(2Z)-3-(3-chlorobenzyl)-2-imino-5,5-dimethylimidazolidin-4-one 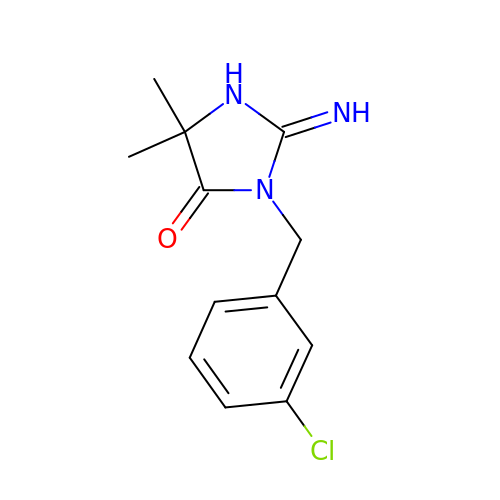| C12 H14 Cl N3 O | NFQQEWLVDJRZJJ-UHFFFAOYSA-N>[2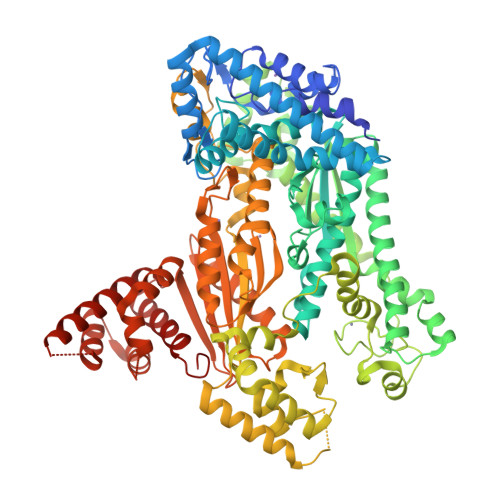x]MHHHHHHENLYFQGAASMVNIKEKLFVYLHDPPDKALKIENHEERSKKILSSGNIQYSRTDKVKQADALSSKTQRFIIRTKENKEPVIDFLGRSSGKYFHVGYPVFIHPISTEIKRYETLEKYIDLGRSNRGERFVNEFLERVSKLEGDVLKEVFEDASNKFKGEESKQWAYIWQFYPVKLKEGVKEFAKSELKLKEEEAEKFAEEFVNLPADTRFPDHAIWTHLDLTSALSVKDPTLLRIKIVPVQPFIANSRKQLDLWASSHLLSMLMYKALEVIVDKFGPEHVIYPSLRDQPFFLKFYLGENIGDEILVANLPNKALAIVSGKEAEKIEEEIKKRIRDFLLQLYREAVDWAVENGVVKVDRSEKDSMLKEAYLKIVREYFTVSITWVSLSEKEDIYQVTENAGLSDEDVKKWLKFAEKKENSRVLERIAIYPLLVKILDSLGERKVTEERFEKSEQLKGWKCHVCGENLAIFGDMYDHDNLKSLWLDEEPLCPMCLIKRYYPVWIRSKTGQKIRFESVVDVALLYKNWRKIFDEKYGKDLVSKAREVSEDFVKDNMLVDSDLYYSSTWESGLSKKLKNKKEIDEEKVKEVVDFLNAAYKEIGNPPKYYAILVMDGDDMGKVISGEVLGEISTRIHPNIRDYVEIPEAKYYSTPQVHVAISQALANFSIREVRSVVKDEGLLIYAGGDDVLAILPVDKALEVAYKIRKEFGKSFENGSLLPGWKLSAGILIVHYKHPLYDALEKARDLLNNKAKNVPGKDTLAIGLLKRSGSYYISLVGWELIRVFYNSELRKKLLEEKGGVGKRFIYHVLREVDTWPKVGIDEMLKFEVIRHIRGRNKEETKELREKIYGEIKDLLEHVRGNNEVEKVRGLFTFLKIITDAEVFP>MNLPTAQEVQGLMARYIELVDVGDIEAIVQMYADDATVENPFGQPPIHGREQIAAFYRQGLGGGKVRACLTGPVRASHNGCGAMPFRVEMVWNGQPCALDVIDVMRFDEHGRIQTMQAYWSEV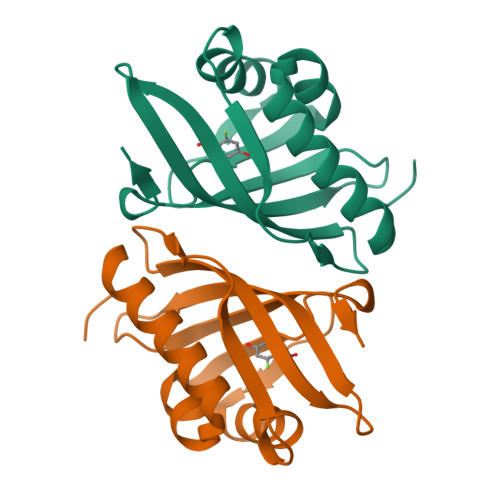NLSVREPQ[2x]>[4x]MDKLAVLYAEHIATLQQRTRTITEREGLEGLVIHSGQAKRQFLDDMYYPFKVNPQFKAWLPVIDNPHCWIVVDGASKPKLIFYRPVDFW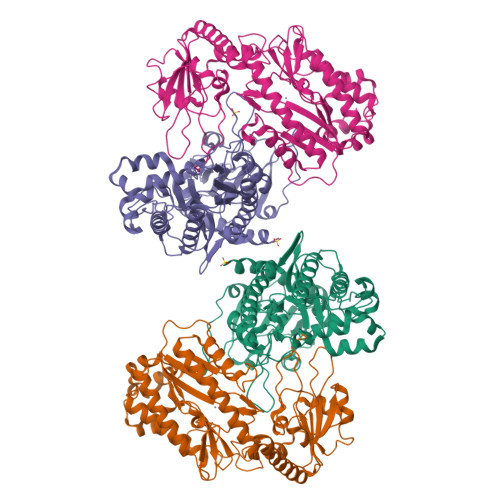HKVPDEPRDFWAEYFDIELLVQPDQVEKLLPYDKANYAYIGEYLEVAQALGFSIMNPEPVMNYLHFHRAYKTQYELECLRQANRIAVEGHKAARDTFFNGGSEFDIQHAYLMATRQSENEMPYGNIVALNENCAILHYTHFEPTAPHTHHSFLIDAGANFNGYAADITRTYDFKKSGEFSDLIQVMTEHQIALGKALKPGLLYGELHLECHQRVAQVLSDFNIVKLPAADIVERGITSTFFPHGLGHHLGLQVHDMGGFMADESGTHQAPPEGHPFLRCTRLIEKNQVFTIEPGLYFIDSLLGDLAQTDNKQFINWEKVEEFKPFGGIRIEDNIIVHEDSLENMTRDLHLDLDHHHHHH ALANYL-PYRIDOXAL-5'-PHOSPHATE | C11 H17 N2 O7 P | 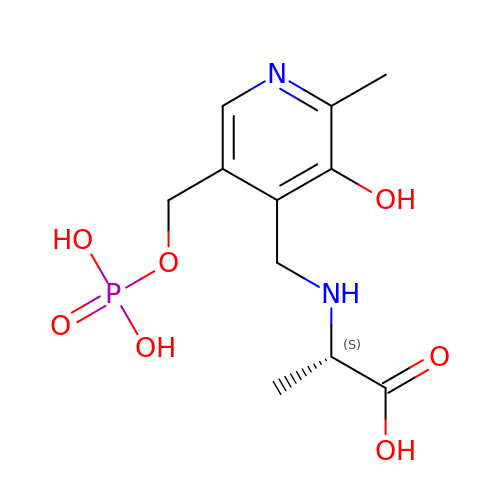WACJCHFWJNNBPR-ZETCQYMHSA-N> SNAGVSDVELRVALPDGTTVTVRVKKNSTTDQVYQAIAAKVGMDSTTVNYFALFEVISHSFVRKLAPNEFPHKLYIQNYTSAVPGTCLTIRKWLFTTEEEILLNDNDLAVTYFFHQAVDDVKKGYIKAEEKSYQLQKLYEQRKMVMYLNMLRTCEGYNEIIFPHCACDSRRKGHVITAISITHFKLHACTEEGQLENQVIAFEWDEMQRWDTDEEGMAFCFEYARGEKKPRWVKIFTPYFNYMHECFERVFCELKWRKEEY;> RGEADLFDSGDIF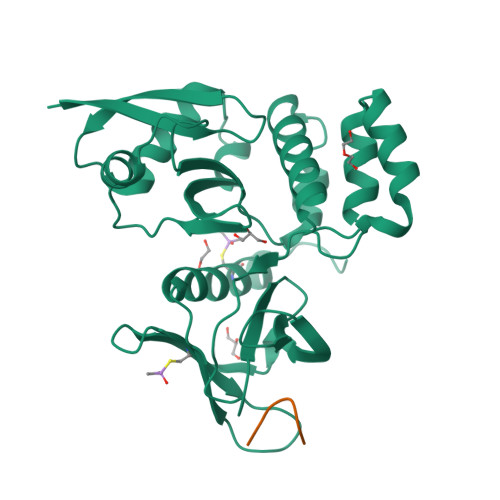STGT> SSKVSEQLKCCSGILKEMFAK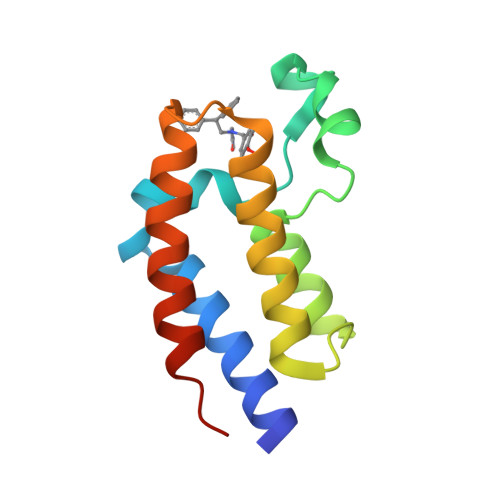KHAAYAWPFYKPVDVEALGLHDYCDIIKHPMDMSTIKSKLEAREYRDAQEFGADVRLMFSNCYKYNPPDHEVVAMARKLQDVFEMRFAKMPDEPEE1-[1-(3,5-dimethoxyphenyl)piperidin-4-yl]-2,3-dimethyl-guanidine | C16 H26 N4 O2 | 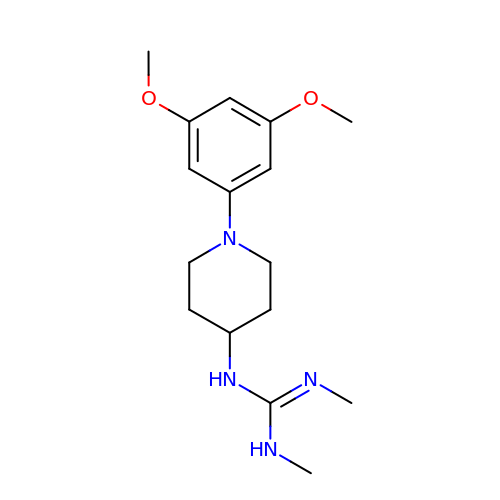NEBYSUCGTBALOK-UHFFFAOYSA-N> FHSGGVAECEGCHTMHNSLGGAVMNSATAQFTTGPMLLQGATQSSSCLNCHQHAGDTGPSSYHISTAEAD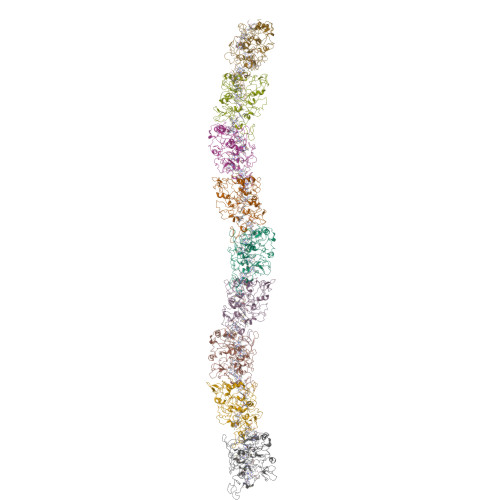MPAGTAPLQMTPGGDFGWVKKTYTWNVRGLNTSEGERKGHNIVAGDYNYVADTTLTTAPGGTYPANQLHCSSCHDPHGKYRRFVDGSIATTGLPIKNSGSYQNSNDPTAWGAVGAYRILGGTGYQPKSLSGSYAFANQVPAAVAPSTYNRTEATTQTRVAYGQGMSEWCANCHTDIHNSAYPTNLRHPAGNGAKFGATIAGLYNSYKKSGDLTGTQASAYLSLAPFEEGTADYTVLKGHAKIDDTALTGADATSNVNCLSCHRAHASGFDSMTRFNLAYEFTTIADASGNSIYGTDPNTSSLQGRSVNEMTAAYYGRTADKFAPYQRALCNKCHAKD> MDISSWFESIHVFL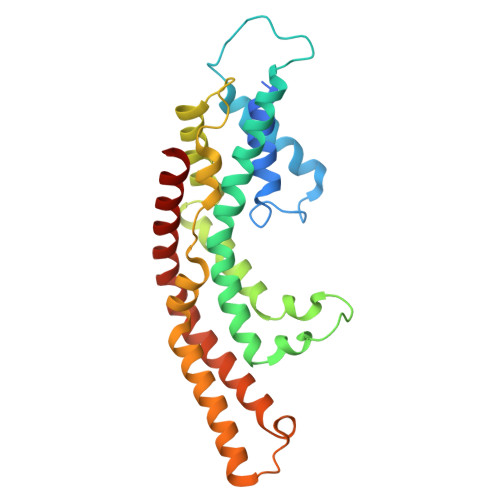ILLNGVFFRLAPLFFFLPFLNNGIISPSIRIPVIFLVASGLITSGKVDIGSSVFEHVYFLMFKEIIVGLLLSFCLSLPFWIFHAVGSIIDNQRGATLSSSIDPANGVDTSELAKFFNLFSAVVFLYSGGMVFILESIQLSYNICPLFSQCSFRISNILTFLTLLASQAVILASPVMIVLLLSEVLLGVLSRFAPQMNAFSVSLTIKSLLAIFIIFICSSTIYFSKVQFFLGEHKFFTNLFVR> TSSDTQNNKTLAAMKNFAEQYAKRTDTYFCSDLSVTAVVIEGLARHKEELGSPLCPCRHYEDKEAE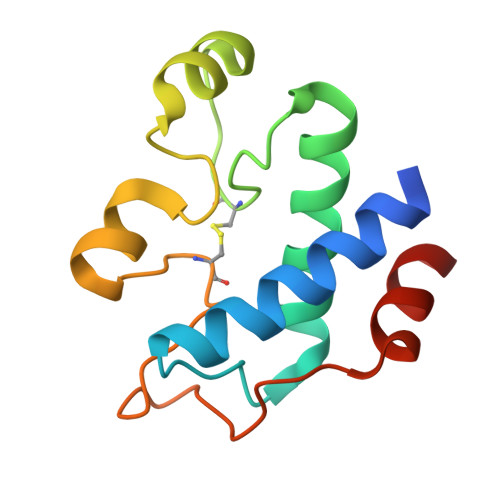VKNTFWNCPCVPMRERKECHCMLFLTPDNDFAGDAQDIPMETLEEVKASMA>[2x]MTQCYAEITGWGKCLPPATLSNHDLSTFLDTSD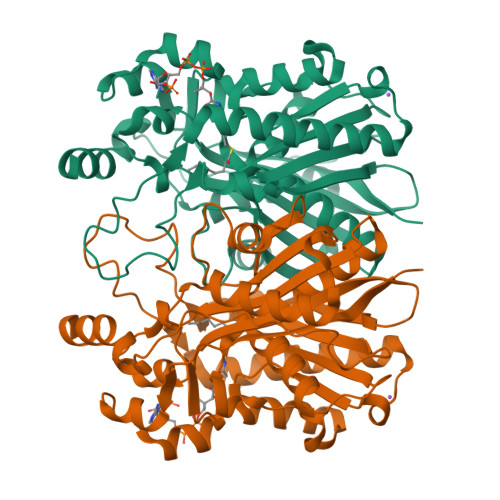EWIQSRTGIEQRRISHVNTSDLATVAAQHAIACAGVSVEEIDLIIVATCSPDSLIPNIASRVQQNLGIPSAAAFDLNAAATGFLYGLETATRLMQASHYRHALVIGAERLSFYLDWTKRDTAVLFGDGAGAVVLSKTEQKVGLQDAQIGCDAQGRDILAVPKFGTAMDRFDADNGYWAFDFVGKEIFKRAVRGMGAAAQQVLARSGLSTEEIDVVIPHQANIRIIQTLCDLAGIAQDKAFVNIHRYGNTSAATVPIALCEALEQGKIKPHDDLLVAAFGAGLTWGAGHIRWGERITPLGKSDAQLPSCDHTALDLLSKAIEHCKRHQSE> GSHMSLAIDLEVKQDVLIVRLSGELDHHTAEELREQVTDVLENRAIRHIVLNLGQLTFMDASGLGVILGRYKQIKNVGGQMVVCAVSPAVKRLFDMSGLFKIIRVEADEQFA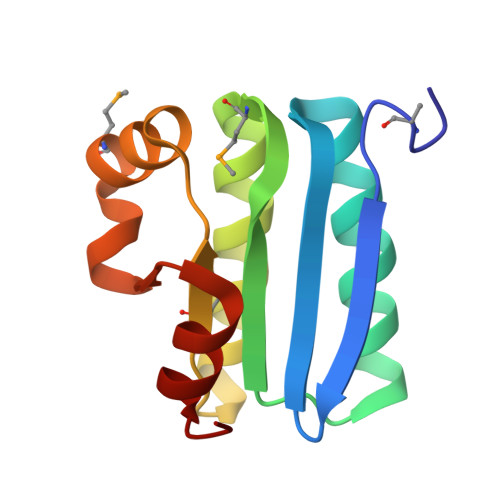LQALGVA>[2x]GPLGSDSRQMTELLDSEQRQGLMIEQHVEAELANDPPNDLMWWRRLFRAIDKWAPPGQRLLLVTTEGRVIGAERSEMQIIRNFIGQADNADHPQKKKYGRVELVGPFSVRDGEDNYQLYLIRPASSSQSDFINLLFDR

CpxA is the sensor kinase of the CpxRA system, a conserved Gram-negative envelope stress response that responds to perturbations to envelope protein homeostasis. Instead, CpxA senses a wide variety of cues that result from envelope stress, especially those arising from misfolded proteins that affect inner membrane integrity. While extracytoplasmic sensor domains adopt a variety of folds, many sensor kinases (and other sensory proteins such as chemotaxis proteins) possess Per-ARNT-Sim (PAS)-like domains in this region. While CpxA contains a PAS domain that is largely similar to the PAS folds of other sensor kinases, CpxA’s “non-canonical” dimer structure regulates its ability to sense periplasmic triggers; diverse inputs that disrupt the stability of the CpxA-SD dimer appear to activate CpxA kinase activity.

Like CpxA in Vibrio parahaemolyticus (CpxA-SDVib), E. coli CpxA-SD (CpxA-SDEC) adopts a PAS-like fold with each globular domain consisting of three α-helices surrounding a five-stranded antiparallel β-sheet in the canonical 2-5-1-4-3 topology. Like other extracytoplasmic PAS domains, CpxA-SD contains a long N-terminal helix (α1). However, this helix does not form the extreme N terminus of the structure, instead containing an N-cap motif at its N terminus and an extended tail region that folds against the β3 strand of the main PAS β-sheet (see later in Results for further discussion of this region). Overall, the monomer structure of CpxA-SDEC is similar to that of the CpxA-SDVib, with an RMSD of 2.9 Å over 108 atoms. While most of these are hydrophobes buried within the PAS domain, asparagine 107 (N107), lysine 121 (K121), and tyrosine 123 (Y123) are notable exceptions. These residues are also located within the deleted region of the constitutively activated and signal blind cpxA24 allele (Δ92–123) and form a hydrogen bond network connecting the α3 helix and β3 strand in our crystal structure. The asymmetric unit of the crystal provided a dimer structure of CpxA-SD where the main dimer interface centers around its ɑ1 helices, which cross each other roughly perpendicularly. In line with this, mutation of the M48 residue (M48K), which lies at the main dimer interface of this structure, did not lead to significant changes in the activation of CpxA or its ability to sense alkaline pH or NlpE overexpression, and CpxA M48K was expressed to similar levels as WT CpxA. This was surprising given the importance of sensor kinase dimerization and led us to conclude that this dimer orientation was likely a crystallographic artifact.>GHMPLLSASIVSAPVVTSETYVDIPGLYLDVAKAGIRDGKLQV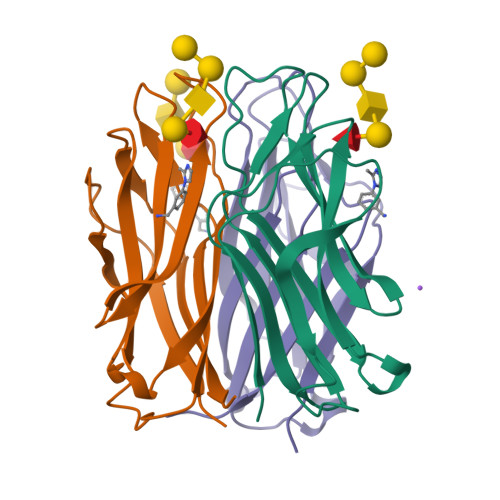ILNVPTPYATGNNFPGIYFAIATNQGVVADGCFTYSSKVPESTGRMPFTLVATIDVGSGVTFVKGQWKSVRGSAMHIDSYASLSAIWGTAA[3x]> ARAPSVSAKPGPALWPLPLSVKMTPNLLHLAPENFYISHSPNSTAGPSCTLLEEAFRRYHGYIFGFYKWHHEPAEFQAKTQVQQLLVSITLQSECDAFPNISSDESYTLLVKEPVAVLKANRVWGALRGLETFSQLVYQDSYGTFTINESTIIDSPRFSHRGILIDTSRHYLPVKIILKTLDAMAFNKFNVLHWHIVDDQSFPYQSITFPELSNKGSYSLSHVYTPNDVRMVIEYARLRGIRVLPEFDTPGHTLSWGKGQKDLLTPCYSGSEPLDSFGPINPTLNTTYSFLTTFFKEISEVFPDQFIHLGGDEVEFKCWESNPKIQDFMRQKGFGTDFKKLESFYIQKVLDIIATINKGSIVWQEVFDDKAKLAPGTIVEVWKDSAYPEELSRVTASGFPVILSAPWYLNRISYGQDWRKYY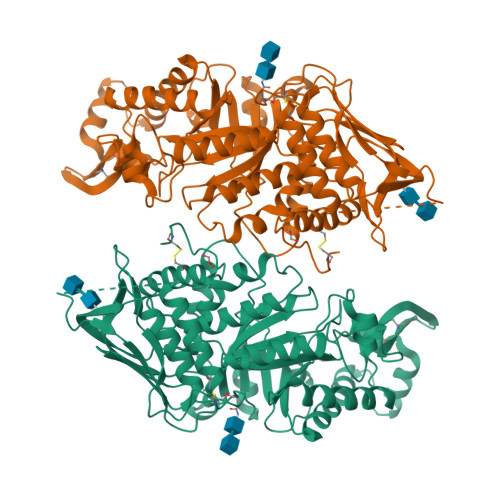KVEPLDFGGTQKQKQLFIGGEACLWGEYVDATNLTPRLWPRASAVGERLWSSKDVRDMDDAYDRLTRHRCRMVERGIAAQPLYAGYCNHENM> MTAPILLLDGASMWFRSYFGVPSSIKAPDGRPVNAVRGFIDAISTLVTREKPRRLVVCRDDDWRPQWRVDLIPSYKAHRVAEPEPDGVPDIEEVPDDLTPQVNMILELLDAFGIPTAGAAGFEADDVLGTLSAREERDPVVVVSGDRNLLQLVRDEPAPQVRVLYLGRGLAKATKWGPAEVAEQYGVPLDRAGTAYAELALL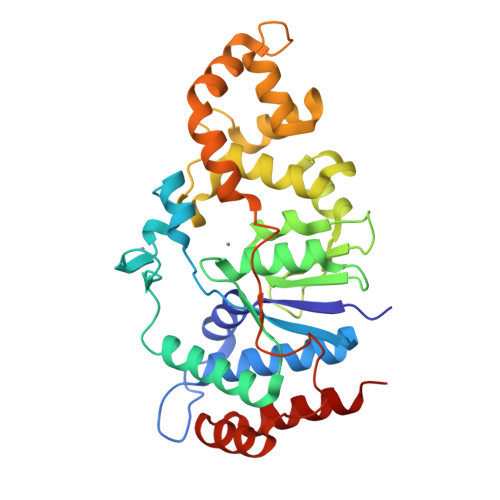RGDPSDGLPGVAGIGEKTAASLLAKHGSLQNILDAAHDPKSGLSKAHRTKLLGAVDYIAAAETVVRVATDAPVTFSTPTDTLPLAAGDPARVAELAAAYGVSSSISRLQTALDQLPD> SNAMPDIFQQEARGWLRCGAPPFAGAVAGLTTKHGGESKGPFASLNMGLHVGDDRTDVVNNRRRLAEWLAFPLERWVCCEQVHGADIQKVTKSDRGNGAQDFATAVPGVDGLYTDEAGVLLALCFADCVPIYFVAPSAGLVGLAHAGWRGTAGGIAGHMVWLWQTREHIAPSDIYVAIGPAIGPCCYTVDDRVVDSLRPTLPPESPLPWRETSPGQYALDLKEANRLQLLAAGVPNSHIYVSERCTSCEEALFFSHRRDRGTT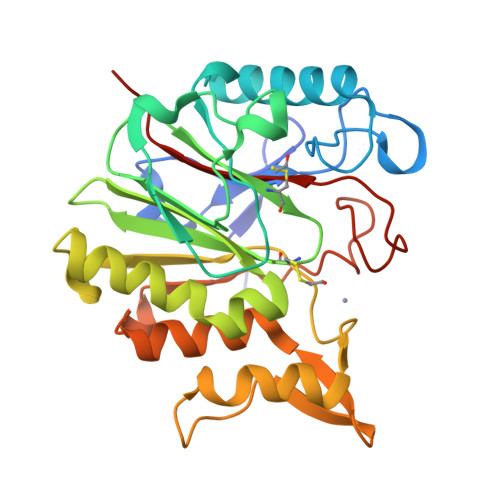GRMLAFIGRREEWT5-methyl-6-{[4-(trifluoromethyl)phenyl]sulfanyl}thieno[2,3-d]pyrimidine-2,4-diamine 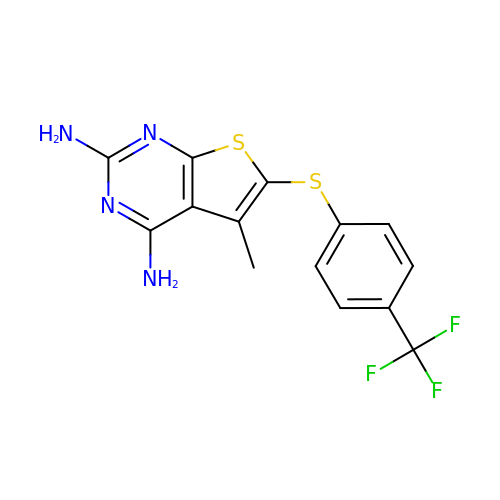| C14 H11 F3 N4 S2 | VWQMUQCLRMRITR-UHFFFAOYSA-N>MQLVLAAKYIGAGISTIGLLGAGIGIAIVFAALINGVSRNPSIKDTVFPMAILGFALSEATGLFCLMVSFLLLFGV[20x];>[2x]MPQLVPFYFMNQLTYGFLLMITLLILFSQFFLPMILRLYVSRLFISKL;>ASTKAQPTEVSSILEERIKGVSDEANLNETGRVLAVGDGIARVFGLNNIQAEELVEFSSGVKGMALNLEPGQVGIVLFGSDRLVKEGELVKRTGNIVDVPVGPGLLGRVVDALGNPIDGKGPIDAAGRSRAQVKAPGILPRRSVHEPVQTGLKAVDALVPIGRGQRELIIGDRQTGKTAVALDTILNQKRWNNGSDESKKLYCVYVAVGQKRSTVAQLVQTLEQHDAMKYSIIVAATASEAAPLQYLAPFTAASIGEWFRDNGKHALIVYDDLSKQAVAYRQLSLLLRRPPGREAYPGDVFYLHSRLLERAAKLSEKEGSGSLTALPVIETQGGDVSAYIPTNVISITDGQIFLEAELFYKGIRPAINVGLSVSRVGSAAQVKALKQVAGSLKLFLAQYREVAAFAQFGSDLDASTKQTLVRGERLTQLLKQNQYSPLATEEQVPLIYAGVNGHLDGIELSRIGEFESSFLSYLKSNHNELLTEIREKGELSKELLASLKSATESFVATF[6x];>ASAAQSTPITGKVTAVIGAIVDVHFEQ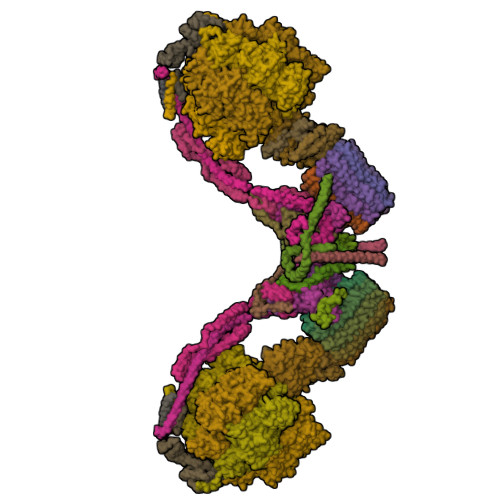SELPAILNALEIKTPQGKLVLEVAQHLGENTVRTIAMDGTEGLVRGEKVLDTGGPISVPVGRETLGRIINVIGEPIDERGPIKSKLRKPIHADPPSFAEQSTSAEILETGIKVVDLLAPYARGGKIGLFGGAGVGKTVFIQELINNIAKAHGGFSVFTGVGERTREGNDLYREMKETGVINLEGESKVALVFGQMNEPPGARARVALTGLTIAEYFRDEEGQDVLLFIDNIFRFTQAGSEVSALLGRIPSAVGYQPTLATDMGLLQERITTTKKGSVTSVQAVYVPADDLTDPAPATTFAHLDATTVLSRGISELGIYPAVDPLDSKSRLLDAAVVGQEHYDVASKVQETLQTYKSLQDIIAILGMDELSEQDKLTVERARKIQRFLSQPFAVAEVFTGIPGKLVRLKDTVASFKAVLEGKYDNIPEHAFYMVGGIEDVVAKAEKLAAEAN[6x];>[2x]ATLKEVEMRLKSIKNIEKITKTMKIVASTRLSKAEKAKISAKKMDEAEQLFYKNAETKNLDVEATETGAPKELIVAITSDKGLCGSIHSQLAKAVRRHLNDQPNADIVTIGDKIKMQLLRTHPNNIKLSINGIGKDAPTFQESALIADKLLSVMKAGTYPKISIFYNDPVSSLSFEPSEKPIFNAKTIEQSPSFGKFEIDTDANVPRDLFEYTLANQMLTAMAQGYAAEISARRNAMDNASKNAGDMINRYSILYNRTRQAVITNELVDIITGASSLG;>AEAAAASSGLKLQFALPHETLYSGSEVTQVNLPAKSGRIGVLANHVPTVEQLLPGVVEVMEGSNSKKFFISGGFATVQPDSQLCVTAIEAFPLESFSQENIKNLLAEAKKNVSSSDAREAAEAAIQVEVLENLQSVLK[2x];>[2x]SAWRKAGMSYAAYLNVAAQAIRSSLKTELQTASVTNRSQTDAFYTQYKNGTAASEPTPMTK;>ASKAAAPPPVRLFGVEGTYATALYQAAAKNSSIDAAFQSLQKVESTVKKNPKLGHLLLNPALSLKDRNSVIDAIVETHKNLDGYVVNLLKVLSENNRLGCFEKIASDFGVLNDAHNGLLKGTVTSAEPLDPKSFKRIEKALSASKLVGQGKSLKLENVVKPEIKGGLIVELGDKTVDLSISTKIQKLNKVLEDSI[2x];>[2x]SPLDQFEIRTLFGLQSSFIDLSCLNLTTFSLYTIIVLLVITSLYTLTNNNNKIIGSRWLISQEAIYDTIMNMTKGQIGGKNWGLYFPMIFTLFMFIFIANLISMIPYSFALSAHLVFIISLSIVIWLGNTILGLYKHGWVFFSLFVPAGTPLPLVPLLVIIETLSYFARAISLGLRLGSNILAGHLLMVILAGLTFNFMLINLFTLVFGFVPLAMILAIMMLEFAIGIIQGYVWAILTASYLKDAVYLH;>MSSTPEKQTDPKAKANSIINAIPGNNILTKTGVLGTSAAAVIYAISNELYVINDESILLLTFLGFTGLVAKYLAPAYKDFADARMKKVSDVLNASRNKHVEAVKDRIDSVSQLQNVAETTKVLFDVSKETVELESEAFELKQKVELAHEAKAVLDSWVRYEASLRQLEQRQLAKSVISRVQSELGNPKFQEKVLQQSISEIEQLLSKLK[2x];>SLAKSAANKLDWAKVISSLRITGSTATQLSSFKKRNDEARRQLLELQSQPTEVDFSHYRSVLKNTSVIDKIESYVKQYKPVKIDASKQLQVIESFEKHAMTNAKETESLVSKELKDLQSTLDNIQSARPFDELTVDDLTKIKPEIDAKVEEMVKKGKWDVPGYKDRFGNLNVM[2x];>VSTLIPPKVVSSKNIGSAPNAKRIANVVHFYKSLPQGPAPAIKANTRLARYKAKYFDGDNASGKPLWHFALGIIAFGYSMEYYFHLRHHKGAEEH[2x];>[2x]MLKRFPTPILKVYWPFFVAGAAVYYGMSKAADLSSNTKEFINDPRNPRFAKGGKFVEVD;>MGAAYHFMGKAIPPHQLAIGTLGLLGLLVVPNPFKSAKPKTVDIKTDNKDEEKFIENYLKKHSEKQDA[2x]> SEISRQEFQRRRQALVEQMQPGSAALIFAAPEVTRSADSEYPYRQNSDFWYFTGFNEPEAVLVLIK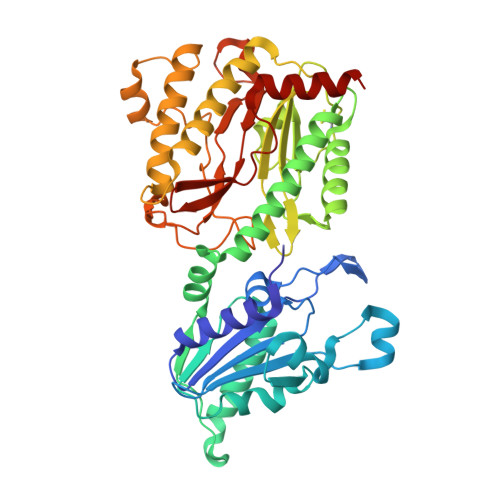SDDTHNHSVLFNRVRDLTAEIWFGRRLGQDAAPEKLGVDRALAFSEINQQLYQLLNGLDVVYHAQGEYAYADVIVNSALEKLRKGSRQNLTAPATMIDWRPVVHEMRLFKSPEEIAVLRRAGEITAMAHTRAMEKCRPGMFEYHLEGEIHHEFNRHGARYPSYNTIVGSGENGCILHYTENECEMRDGDLVLIDAGCEYKGYAGDITRTFPVNGKFTQAQREIYDIVLESLETSLRLYRPGTSILEVTGEVVRIMVSGLVKLGILKGDVDELIAQNAHRPFFMHGLSHWLGLDVHDVGVYGQDRSRILEPGMVLTVAPGLYIAPDAEVPEQYRGIGIRIEDDIVITETGNENLTASVVKKPEEIEALMVAARKQ The eukaryotic translation initiation factor 4E (eIF4E) protein is a vital component of the cap-dependent mechanism for mRNA translation. It binds the 7-methylguanosine (m7G) cap structure present at the 5′ end of mRNA molecules and recruits it as part of the eIF4F assembly which also includes two other partner proteins, eIF4A and eIF4G, to the translational machinery for protein synthesis. We have used a structure-guided approach to rationally develop a set of hydrocarbon stapled-peptides with high binding affinities and residence times against the oncogenic eukaryotic translation initiation factor 4E (eIF4E) protein. Crystal structures of these peptides in complex with eIF4E show that they form specific interactions with a region on the protein-binding interface of eIF4E which is distinct from the other well-established canonical interactions.

The hydrocarbon linker was found to be exposed to the solvent and did not engage with eIF4E. The specific interactions observed in other peptide: eIF4E structures, including a hydrogen-bond and salt-bridge between Y4-P38 and R6-E132 respectively, docking of the sidechain of L9 into a shallow pocket on eIF4E and a hydrogen-bond between the peptide backbone and the W73 side-chain of eIF4E, are all preserved in this crystal structure. In addition to these canonical interactions, we noticed an exposed untapped patch on the surface of eIF4E with potential to be targeted by interactions with the C-terminal end of a modified peptide. This region comprised of residues W73, Y76, N77 and L131, offering aromatic, hydrophobic and hydrogen-bonding properties. Next, molecular dynamics (MD) simulations were carried out on the crystallographic complex of sTIP-05: eIF4E and on a modeled complex of sTIP-06: eIF4E (generated by constructing in silico amino acid changes in the crystal structure of sTIP-05: eIF4E complex). They showed that the patch on eIF4E remained solvent exposed and neither of the 12mer peptides could engage it (Movies S1 and S2†). We hypothesized that a peptide extension at the C-termini may help engage this patch for more efficient target binding.

> MVANPEHYIKHPLQNRWALWFFKNDKSKTWQANLRLISKFDTVEDFWALYNHIQLSSNLMPGCDYSLFKDGIEPMWEDEKNKRGGRWLITLNKQQRRSDLDRFWLETLLCLIGESFDDYSDDVCGAVVNVRAKGDKIAIWTTECENREAVTHIGRVYKERLGLPPKIVIGYQSHADTATKSGSTTKNRFVV>[2x]MKGPAFEFAVAMMKRNASTVKTEYGEFTMLGIYDRWAVLPRHAKPGPTILMNDQEVGVLDAKELVDKDGTNLELTLLKLNRNEK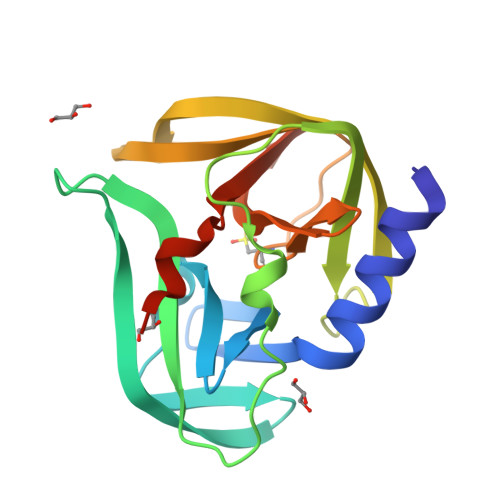FRDIRGFLAREEVEVNEAVLAINTSKFPNMYIPVGQVTDYGFLNLGGTPTKRMLVYNFPTRAGQCGGVLMSTGKVLGIHVGGNGHQGFSAALLRHYFNEEQHHHHHH>MSNKEYRPTLAQLRTFVTIAECKHFGTAATKLSISQPSLSQALVALETGLGVQLIERSTRKVIVTPAGEKLLPFAKSTLDAAESFLSHAKGANGSLTGPLTVGIIPTAAPYILPSMLSIVDEEYPDLEPHIVEDQTKHLLALLRDGAIDVAMMALPSEAPGMKEIPLYDEDFIVVTASDHPFAGRQDLELSALEDLDLLLLDDGHSLHDQIVDLCRRGDINPISSTTAVTRASSLTTVMQLVVAGLGSTLVPISAIPWECTRPGLATANFNSDVTANRRIGLVYRSSSSRAEEFEQFALILQRAFQEAVALAASTGITLKQN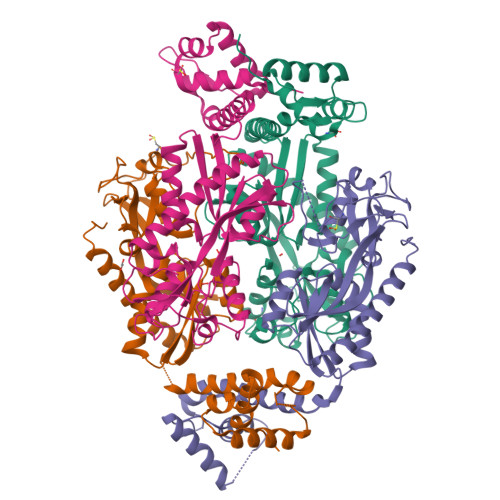VAVAQ[4x]>GSHMKKLILDLDTGVDDTLAISYALGSPEMELIGITGTYGNVLMEQGVRNALAITDLLGHPEVKVYKGLSHASTKDSFEVLPISAFIHGDNGIGDVEIPDSPRKAEDESAVDFIIDSVKKYGKDLVYVPTGPMTNIAAALKKAPEIKDEIGKIVLMGGALTIHGNVNAWTEANISQDPDAADILFRSGAPVTMIGLDVTLQTLLTYKETKQWRDLNTKAGKFLADMTDFYIKAYETTAPHLGGCGLHDPLAVAVAVDPTLVTTLPINMQVDVEGPTRGRTIGDVTRLNDPVKTMQVAVGVDVPRFLNEFMTRISGLAKIAG[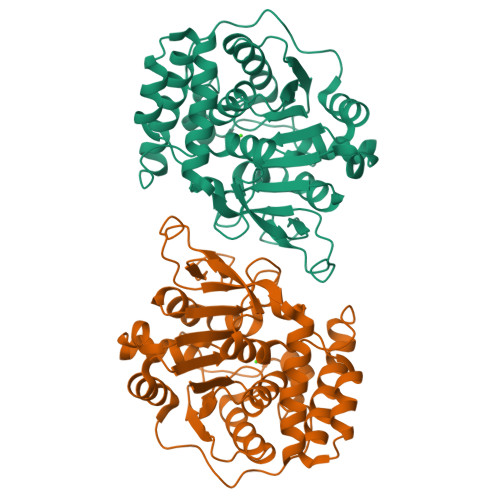18x]> MTMVDREQLFKKALEIKFTQEWGEN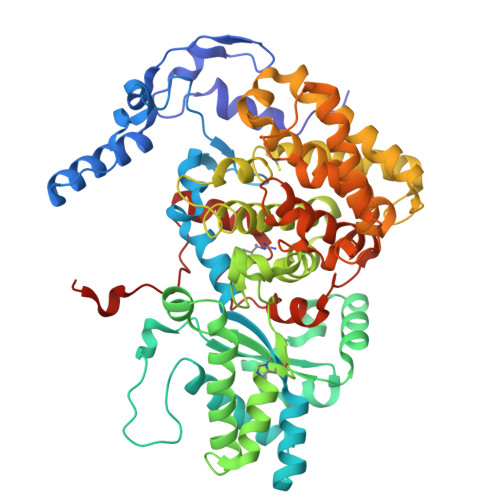KATEVSTDITSKKAKYLRLGTAQSPRKREFEQYGKEIAAKRGLPGYDPKLHLGGIPLGQRQITPYVVSSTDTLCDGDDLHFVNNAAMQQMWDDIRRTVIVGMDLAHETLEKRLGKEVTPETINHYLEVLNHAMPGAAVVQEMMVETHPGLVDDCYVKVFTGDDELADEIDKRFLIDIDKQFGEEKAAQIKAAIGKTTWQAVHVPTIVVRTCDGATTSRWTAMQIGMSFIAAYRMCAGEAAVADLAYAAKHAALVGMGDMLPARRARGPNEPGGLQFGYLADIVQADRVTDDKVKASLEVVAAGAMLYDQIWLGSYMSGGVGFTQYATAAYTNNILDDFSYYGYEYAVDKYGGPAQAPATLETVKDIATETAIYAIEQYEYFPTLLEDQFGGSQRAAVVAAAAGIATGLATGNSQAGLSGWYLAQYLLKEAEGRLGFFGYDLQDQCGAANVFSYQSDEGLPLELRGPNYPNYAMNVGHQGEYAGIASSGHIGRGDAFVVNPLVKVAFADPLLNFDFTQVRKEFAKGAVREFDRCAGERALILPAK(1R,3S,5Z)-4-methylidene-5-[(E)-3-[3-[7,7,7-tris(fluoranyl)-6-oxidanyl-6-(trifluoromethyl)heptyl]phenyl]pent-2-enylidene]cyclohexane-1,3-diol 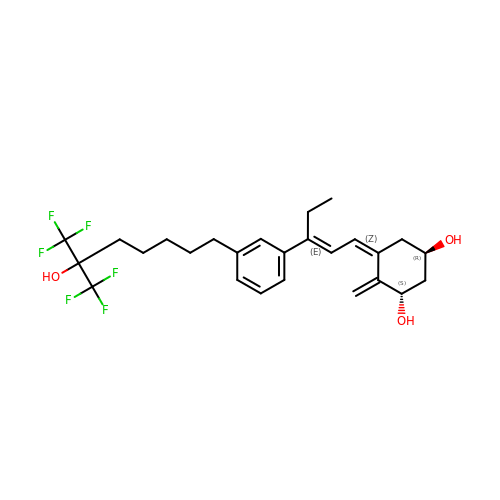| C26 H32 F6 O3 | MARICLVKOFLLAP-JRJKOMHBSA-N>[9x]MRGSHHHHHHGRSLNPLSTPQFDSTDETPASYNLAVRRAAPAVVNVYNRGLNTNSHNQLEIRTLGSGVIMDQRG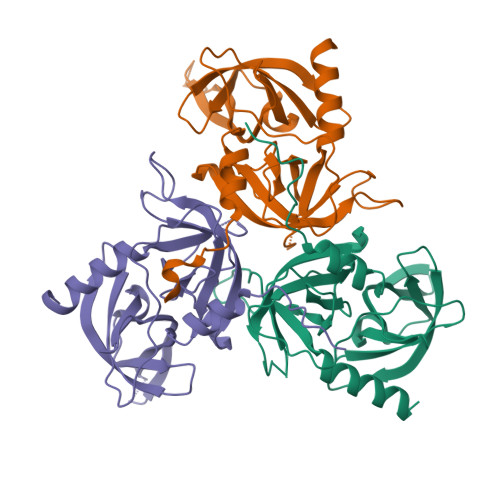YIITNKHVINDADQIIVALQDGRVFEALLVGSDSLTDLAVLKINATGGLPTIPINARRVPHIGDVVLAIGNPYNLGQTITQGIISATGRIGLNPTGRQNFLQTDASINPGNSGGALVNSLGELMGINTLSFDKSNDGETPEGIGFAIPFQLATKIMDKLIRDGRVIR>[4x]MSKSNQKIASIEQLSNNEGIISALAFDQRGALKRMMAKHQTEEPTVAQ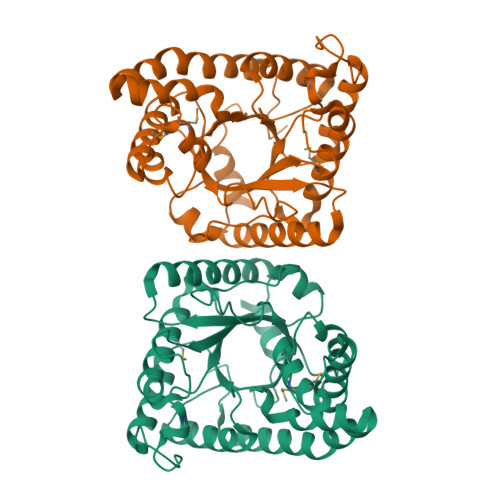IEQLKVLVAEELTQYASSILLDPEYGLPASDARNKDCGLLLAYEKTGYDVNAKGRLPDCLVEWSAKRLKEQGANAVKFLLYYDVDDAEEINIQKKAYIERIGSECVAEDIPFFLEVLTYDDNIPDNGSVEFAKVKPRKVNEAMKLFSEPRFNVDVLKVEVPVNMKYVEGFAEGEVVYTKEEAAQHFKDQDAATHLPYIYLSAGVSAELFQETLKFAHEAGAKFNGVLCGRATWSGAVQVYIEQGEDAAREWLRTTGFKNIDDLNKVLKDTATSWKQRKLEHHHHHH> MRRAVVSSSPPPSYESVMAQATLEVPFVPPRYMAPTEGRNSIRYSELAPQYDTTRVYLVDNKSADIASLNYQNDHSNFLTTVVQNNDFTPAEASTQTINFDERSRWGGDLKTILHTNMPNVNEYMFTSKFKARVMVSRKHPEGVVETDLSQDKLEYEWFEFTLPEGNFSETMTIDLMNNAILENYLQVGRQNGVLESDIGVKFDSRNFKLGWDPVTKLVMPGVYTYEAFHPDVVLLPGCGVD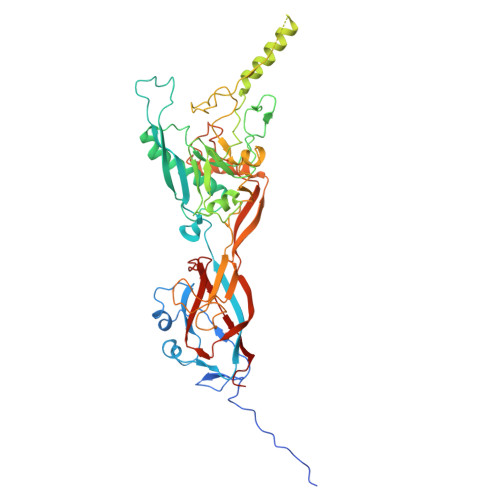FTESRLSNLLGIRKKQPFQEGFRIMYEDLEGGNIPALLDVPKYLESKKKVEDETKNAAAATADTTTRGDTFATPAQETAADKKVEVLPIEKDESGRSYNLIQGTHDTLYRSWYLSYTYGDPEKGVQSWTLLTTPDVTCGAEQVYWSLPDLMQDPVTFRSTQQVSNYPVVGAELMPFRAKSFYNDLAVYSQLIRSYTSLTHVFNRFPDNQILCRPPAPTITTVSENVPALTDHGTLPLRSSIRGVQRVTVTDARRRTCPYVYKALGIVAPRVLSSRTF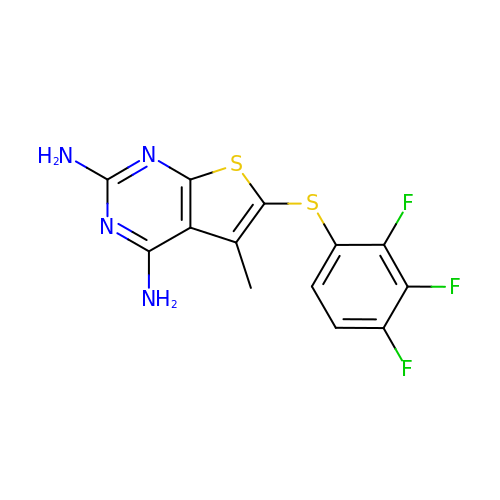5-methyl-6-[(2,3,4-trifluorophenyl)sulfanyl]thieno[2,3-d]pyrimidine-2,4-diamine | C13 H9 F3 N4 S2 | HOYROOKWEBIDCA-UHFFFAOYSA-N> WL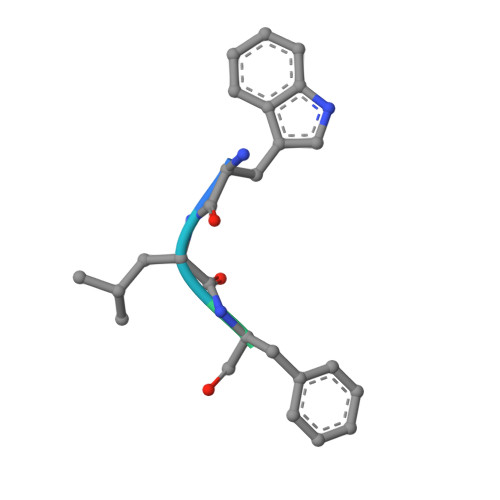FVQRDSKE>MTTADRASEFLGGLFNSLTERGRSLFGLTSSQPMSGDELIALSETLLSRRGEASGVALAASLLAGYEAADEDDKLAFLDALAEQFGPDLAELNTAIEAFRADASAEATGELLRAAEPRRQELIRRLNHAPGGTAALVKMREAVLARIAAHPQLRHVDDDFVHLFTSWFNRGFLVLQRIDWTTPANILEKIIRYEQVHTIHDWDDLRARLAPPDRRCYGFFHPRLVDEPLIFVEVALTKDSPAAIAPLLDLEREPIAASDATTAVFYSISNTQQGLAGISFGNFLIKQVVEEIKRELPNVQTFVTLSPVPGFAKWLKRERDNPDSTLLDASARTALEALDTPNWFDDADTADRLKPIVLQLAAAYFLQAKGPNGRPLDPVARFHLGNGARLDRLNFLGDRSPNGMRQSHGLMVNYLYALGDIEANHEALFERGQIAAASAVRKLVPLEHHHHHH[4x]

Malonyl-coenzyme A decarboxylase (MCD) is found from bacteria to humans, has important roles in regulating fatty acid metabolism and food intake, and is an attractive target for drug discovery. The MCD monomer contains an N-terminal helical domain involved in oligomerization and a C-terminal catalytic domain. Unexpectedly, the MCD catalytic domain is structurally homologous to those of the GCN5-related N-acetyltransferase superfamily, especially the curacin A polyketide synthase catalytic module, with a conserved His-Ser/Thr dyad important for catalysis. The catalytic domain of MCD contains a central eight-stranded, mostly antiparallel β sheet (β1–β8) that is surrounded by at least 11 α helices (α1–α11).

We solved the structure of RpMCD by the selenomethionyl single-wavelength anomalous diffraction method and the structures of AvMCD and CmMCD by molecular replacement. RpMCD and AvMCD are also tetramers in solution, based on multiangle static light scattering studies (data not shown). Like HsMCD, the RpMCD and AvMCD tetramers are also dimer of dimers. However, the relative orientations of the dimers are substantially different. The central cavity of RpMCD tetramer also contains a helical segment (αA′) from the N terminus of two of the monomers. For RpMCD, residues 55–58 in the other monomer of the dimer, in the loop linking the first two helices of the N-terminal domain, approach within ∼10 Å of the expected position of the adenosine group in the active site. Moreover, the loop and the following helix α4 are positioned differently in RpMCD and CmMCD, suggesting that the binding mode of CoA to these MCDs may be somewhat different unless there is a conformational change upon CoA binding in these two enzymes. The 3′ phosphate group on the ribose of CoA is recognized by Arg387 in CurA (equivalent to Asn421 in HsMCD). This residue is equivalent to Arg387 in RpMCD, which may have a similar function. The equivalent residues, His423 and Ser329 in HsMCD and His389 and Ser312 in RpMCD, are strictly conserved among the MCDs. However, this Arg residue is not conserved in RpMCD (Asp404), and in fact, an Asp residue is conserved at this position among the MCDs.>[2x]MGDRVNAQDDDTVVPHQAPLQPAALQQDLTRSADYLLDNVRIGNHRQRYDKYRRYVLLRSSEIFTSLVAIYAHIFSSYWQHFRRFTDQFQAPTGVQLPTFVARVYISTWLHDLYCSIREATRSISPLAFNERYSYELLPYSTEYDPFLAFLSMSIKPTHIQHTPE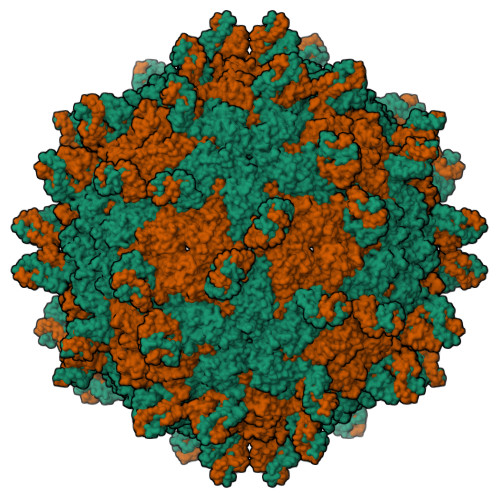NTLWIPILCENYDWDRNEANHNPFGITNFTLNSNLFYGLLAILKERKEFKLSTLTTNTIGRPCWLFDWHDNVQVCAWFPREANFNSQDVTAAYIIGVACTPKLGPSDDDAWKYYASLNSVPTFTPTEPRLTNRRSYGAYEVRTRETENNYFLPDSLLNIIEDFTATGTTQRRKIRRPSATSASTGAAIIIRDTPGTASTATTSTTETEVTFPPVIRTKIRDWYYHSRVILELEDNSRTAALRMFIIA> MPEDQVGKLEATENTISAMAAAAAEQQQFYLLLGNLLSPDNVVRKQAEETYENIPGQSKITFLLQAIRNTTAAEEARQMAAVLLRRLLSSAFDEVYPALPSDVQTAIKSELLMIIQMETQSSMRKKVCDIAAELARNLIDEDGNNQWPEGLKFLFDSVSSQNVGLREAALHIFWNFPGIFGNQQQHYLDVIKRMLVQCMQDQEHPSIRTLSARATAAFILANEHNVALFKHFADLLPGFLQAVNDSCYQNDDSVLKSLVEIADTVPKYLRPHLEATLQLSLKLCGDTSLNNMQR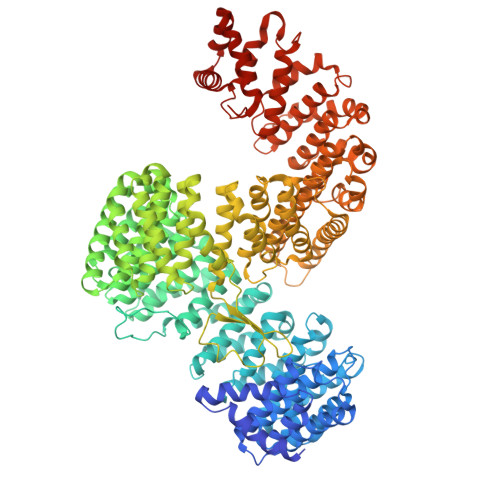QLALEVIVTLSETAAAMLRKHTNIVAQTIPQMLAMMVDLEEDEDWANADELEDDDFDSNAVAGESALDRMACGLGGKLVLPMIKEHIMQMLQNPDWKYRHAGLMALSAIGEGCHQQMEGILNEIVNFVLLFLQDPHPRVRYAACNAVGQMATDFAPGFQKKFHEKVIAALLQTMEDQGNQRVQAHAAAALINFTEDCPKSLLIPYLDNLVKHLHSIMVLKLQELIQKGTKLVLEQVVTSIASVADTAEEKFVPYYDLFMPSLKHIVENAVQKELRLLRGKTIECISLIGLAVGKEKFMQDASDVMQLLLKTQTDFNDMEDDDPQISYMISAWARMCKILGKEFQQYLPVVMGPLMKTASIKPEVALLDTQDMENMSDDDGWEFVNLGDQQSFGIKTAGLEEKSTACQMLVCYAKELKEGFVEYTEQVVKLMVPLLKFYFHDGVRVAAAESMPLLLECARVRGPEYLTQMWHFMCDALIKAIGTEPDSDVLSEIMHSFAKCIEVMGDGCLNNEHFEELGGILKAKLEEHFKNQELRQVKRQDEDYDEQVEESLQDEDDNDVYILTKVSDILHSIFSSYKEKVLPWFEQLLPLIVNLICPHRPWPDRQWGLCIFDDVIEHCSPASFKYAEYFLRPMLQYVCDNSPEVRQAAAYGLGVMAQYGGDNYRPFCTEALPLLVRVIQSADSKTKENVNATENCISAVGKIMKFKPDCVNVEEVLPHWLSWLPLHEDKEEAVQTFNYLCDLIESNHPIVLGPNNTNLPKIFSIIAEGEMHEAIKHEDPCAKRLANVVRQVQTSGGLWTECIAQLSPEQQAAIQELLNSA> AKVVKFSYMWTINNFSFCREEMGEVIKSSTFSSGANDKLKWCLRVNPKGLDEESKDYLSLYLLLVSCPKSEVRAKF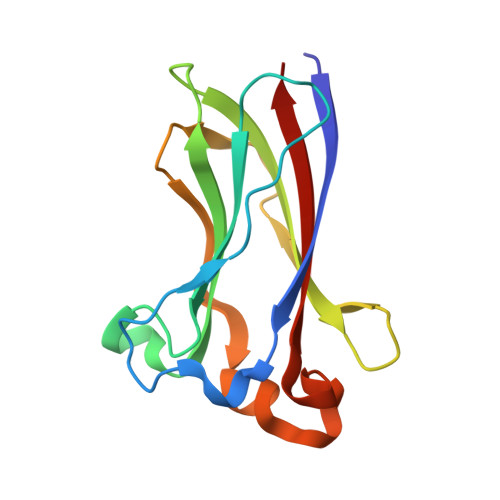KFSILNAKGEETKAMESQRAYRFVQGKDWGFKKFIRRDFLLDEANGLLPDDKLTLFCEVSVVQD> MRGSHHHHHHGMASVFADSLFSDRFNRIDRLFSQLTGDTPVAATPAYDLQKRDANNYLLTVSVPGWKEEELEIETVGGNLNITGKHTEETVEDQTHWIYRGIRKADFQLSFSLPEHAKVNNAKLEQGLLLVEIYQEIPESEKPKKIAIES

Small Heat Shock Proteins (sHSPs) are ATP-independent chaperones which prevent irreversible protein aggregation by binding to misfolded substrate proteins. Most sHSPs exist as large oligomers which undergo drastic rearrangement or dissociation into dimers upon activation during stress, in order to execute their chaperone function. Aggregation Suppressing Protein A (AgsA), an sHSP from the pathogenic bacterium Salmonella enterica has been reported to form dynamic oligomers. In line with the current understanding of sHSP structure and function, our results show that in vivo, the wild type protein exists in an equilibrium between two oligomeric states: 18-mer and 24-mer.

The core ACD fragment of AgsA:His-DD crystallized as a symmetric dimer in the space group P41212. Mass spectrometry of the crystals revealed that the full length protein (size 17.1 kDa, 150 amino acids) had degraded in the crystallization condition to a fragment with mass 12.7 kDa, which corresponds to residues 35–147. Continuous electron density could be traced for residues 40–132, and the monomer adopts an α-crystallin-like fold, with residues 83–103 forming a long loop which separates two β-sheets. Residues 93–98 of this loop in subunit 1, form part of a β-sheet in subunit 2. In the AgsA:His-DD dimer, this groove is occupied by the dimerization loop of a subunit belonging to a neighbouring dimer. This interaction buries 434 Å2 of surface area and involves five hydrogen bonds and one salt bridge. The hydrophobic cleft is known to be a substrate binding site15 and the binding of the eight residue stretch from the dimerization loop may represent the interaction between a sHSP and its substrate. Unlike all other non-metazoan sHSP dimers which form 3–4 intra-dimer salt bridges, there are no salt bridges between the two subunits of the AgsA ACD dimer. Structural and sequence alignments reveal that in AgsA, the equivalent residues to Arginine and Glutamate are Leu106 and Gly98, respectively. Leu106 of subunit 1 makes no contact with the dimerization loop of subunit 2, whereas Gly98 of subunit 1 participates in the formation of two hydrogen bonds, one each with Tyr44 and Asp45 on the β2 strand of subunit 2.> KQLMLDGPKSEPADPFISLLMDPLEESVGKVVNHIAQLFEEASKNEGDESLVLRSQLGYQLFFLIVRSLADGKREVSKKILSGIPTSVRAEVFPGLQRSVYKSAVFLGNHIIQVLLGSKKSFEDWDVVGVAKDLESAWKRRAIAELIKKFQVSILEQCFDKPVPLIPQSPLNNDAVIDNVNKALQFALWLTEFYGSENETEALGELRFLDST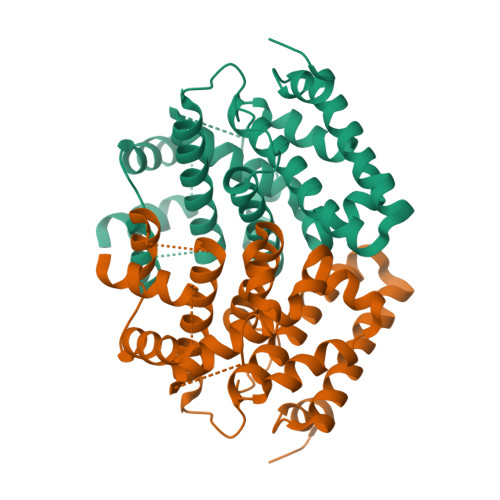SKNLLVDSFKKFVQGINSKTHVTRIVESLEK>[4x]VSELSVATGAVSTASSSIPMPAGVNPADLAAELAAVVTESVDEDYLLYECDGQWVLAAGVQAMVELDSDELRVIRDGVTRRQQWSGRPGAALGEAVDRLLLETDQAFGWVAFEFGVHRYGLQ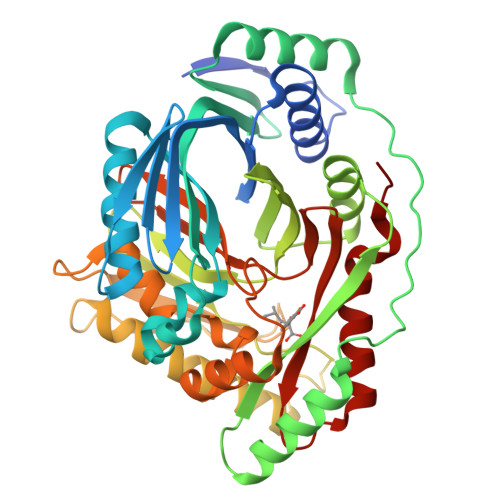QRLAPHTPLARVFSPRTRIMVSEKEIRLFDAGIRHREAIDRLLATGVREVPQSRSVDVSDDPSGFRRRVAVAVDEIAAGRYHKVILSRCVEVPFAIDFPLTYRLGRRHNTPVRSFLLQLGGIRALGYSPELVTAVRADGVVITEPLAGTRALGRGPAIDRLARDDLESNSKEIVEHAISVRSSLEEITDIAEPGSAAVIDFMTVRERGSVQHLGSTIRARLDPSSDRMAALEALFPAVTASGIPKAAGVEAIFRLDECPRGLYSGAVVMLSADGGLDAALTLRAAYQVGGRTWLRAGAGIIEESEPEREFEETCEKLSTLTPYLVARQ>HHHHHHHTPSTQHSRPLTSEAFAALGAPALVYVRPIKAAEILADAPEGVEDLDLSPDQTLYAVCRADGERLAVLIDRDTAIAAALAHELA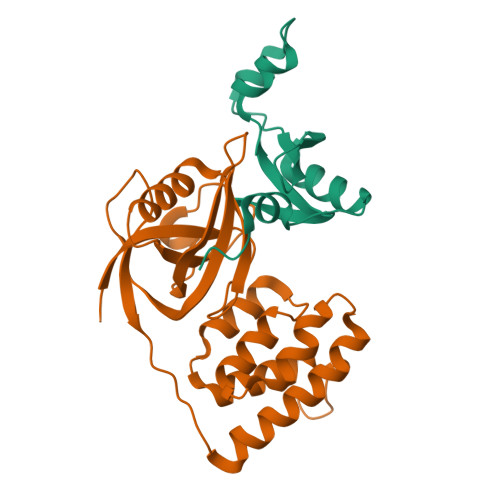PVSVH[2x];>[2x]SELRTLPVLPLRDIVVFPHMVVPLFVGRDKSVRALEEVMRGDKQILLVTQKNSADDDPAPGDIFEVGVLATVLQLLKLPDGTVKVLVEGKARAAVVSFTDQESYYEAQIGEVSEDDGAGPEAEALSRAVVEQFENYVKLNKKVPPEALASIPQIAEPGKLADSIAAHLSVKIGDKQNLLEIFDVVKRLEKVFALMEGEISVLQVEK>[2x]MNKPQTIYEKLGGENAMKAAVPLFYKKVLADERVKHFFKNTDMDHETKQQTDFLTM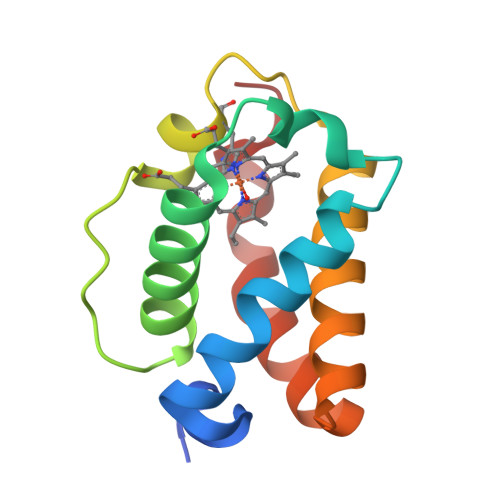LLGGPNHYKGKNMTEAHKGMNLQNLHFDAIIENLAATLKELGVTDAVINEAAKVIEHTRKDMLGK>INQVRPKLPLLKILHAAGAQGEMFTVKEVMHYLGQYIMVKQLYDAAAQHMVYCGGDLLGELLGRQSFSVKDP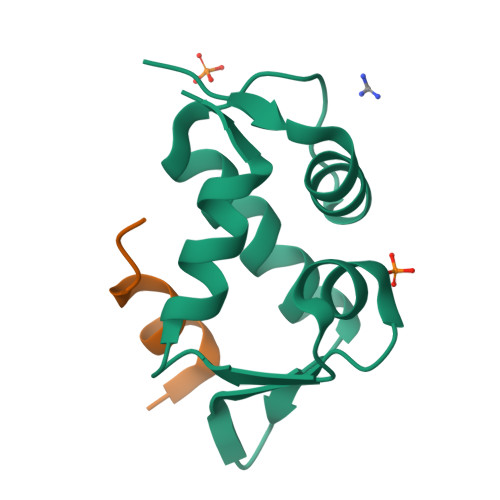SPLYDMLRKNLVT[2x];>TSFAEYWNLLSP[2x]>[2x]GPGGSGGMKPQIRNMVEPMDPRTFVSNFNNRPILSGLDTVWLCCEVKTKDPSGPPLDAKIFQGKVYPKAKYHPEMRFLRWFHKWRQLHHDQEYKVTWYVSWSPCTRCANSVATFLAKDPKVTLTIFVARLYYFWDPDYQQALRILAEAGATMKIMNYNEFQDCWNKFVDGRGKPFKPWNNLPKHYTLLQATLGELLRHLMDPGTFTSNFNNKPWVSGQHETYLCYKVERLHNDTWVPLNQHRGFLRNQAPNIHGFPKGRHAQLCFLDLIPFWKLDGQQYRVTCFTSWSPCFSCAQEMAKFISNNEHVSLCIFAARIYDDQGRYQEGLRTLHRDGAKIAMMNYSEFEYCWDTFVDRQGRPFQPWDGLDEHSQALSGRLRAILQNQGN

APOBEC3s (A3s) are an APOBEC subfamily in mammals that restrict viruses, including retroviruses, endogenous retroelements, Hepatitis B virus, and Epstein-Barr virus. The double-domain A3G, A3F, A3D, and single-domain A3H (haplotypes II, V, and VII) are active in restricting HIV-1 through deaminase-dependent and independent modes, with A3G being most potent among them. For the double-domain A3s, the deaminase activity resides only on CD2, but the catalytically inactive CD1 is important for regulating nucleic acid binding, processivity, oligomerization, packaging into HIV virion, and effective anti-HIV activity. In order to understand the structural basis of domain organization and molecular regulation of the complex biological functions of A3G, we determined the double-domain structure of rA3G.

The E/Q construct was crystallized in different pH and salt conditions but consistently showed the same structure and dimerization via CD1-CD1 interactions, primarily through direct packing of several residues on h6 (K180, L184, A187), loop 1 (I26) and loop 7 (F126, W127) from both subunits. While the FKL structure shows a canonical fold of its CD2 domain, the E/Q structure shows significant alteration in CD2 conformation, with major changes on helix 2 (h2), loop 3, loop 4, and the Zn-active center. The long h2 of the CD2 in the FKL structure has become a short 310 helix (h2′) in the E/Q structure, resulting in a disordered 14-residue stretch spanning parts of loop 3 and h2 (residues A246 to E259). The shift to a short 310 h2 and extended random coil structure is necessary to avoid clashing in this tight packing conformation. However, this also disrupts the conformation of the CD2 Zn-active center within the regions of h2 and loop 3 that become disordered, resulting in no Zn-coordination. When aligning the FKL and E/Q structures via their CD1 domain, the CD2 domain of the E/Q structure shows a rotation of ~29° compared with the CD2 of FKL structure, causing the E/Q CD2 domain to shift ~15 Å downward and ~8 Å toward CD1, and resulting in a much closer packing interaction with CD1. In the E/Q structure, the two domains interact mainly through h3, h4, and h6 of CD1 with h2′, β2, loop 4 and loop 10 of CD2. Additionally, E/Q* carrying individual mutations F126Y, K180S/L184S, or CD2Δloop3 (as in FKL structure) are all active, even though the activity of the FKL* construct (with E259A reverted back to E259) with the combined mutations is less than E/Q* and WT. These results suggest that even though the crystallized E/Q structure, lacking Zn in the CD2 domain, represents a catalytically inactive A3G structural state, reverting the catalytic residue back to E259 can fully restore its deaminase activity comparable to WT. Full-length rA3G dimerizes through a hydrophobic CD1-CD1 protein interface and dimerization generates an area with intensified positive electrostatic potentials (PEP).> AAGSVPATNQLVDYVVNVGVGSPATTYSLLVDTGSSNTWLGADKSYVKTSTSSATSDKVSVTYGSGSFSGTEYTDTVTLGSLTIPKQSIGVASRDSGFDGVDGILGVGPVDLTVGTLSPHTSTSIPTVTDNLFSQGTIPTNLLAVSFEPTTSESSTNGELTFGATDSSKYTGSITYTPITSTSPASAYWGINQSIRYGSSTSILSSTAGIVDTGTTLTLIASDAFAKYKKATGAVADNNTGLLRLTTAQYANLQSLFFTIGGQTFELTAN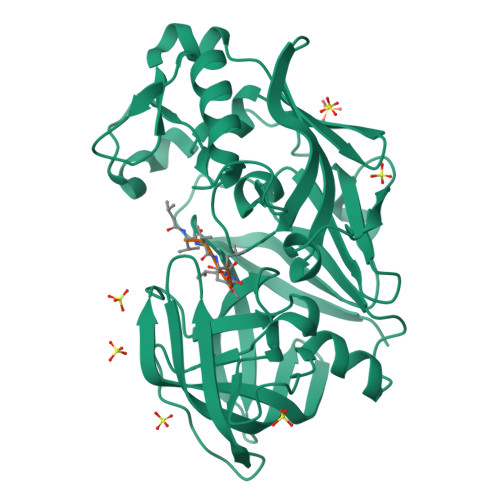AQIWPRNLNTAIGGSASSVYLIVGDLGSDSGEGLDFINGLTFLERFYSVYDTTNKRLGLATTSFTTATSN> SMGYGNGVLIPHTPIAV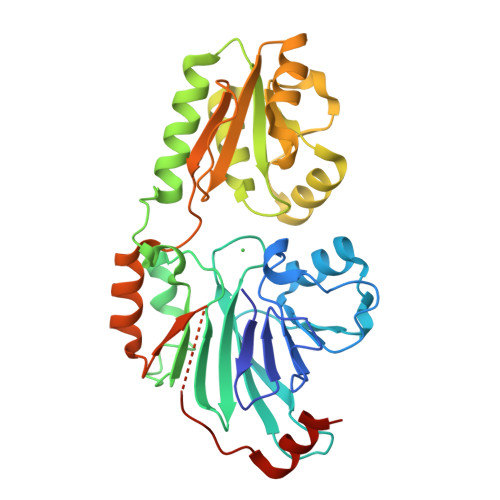DFWSLRRAGTARLFFLSHMHSDHTVGLSSTWARPLYCSPITAHLLHRYLQVSKQWIQALEVGESHVLPLDEIGQETMTVTLLDANHCPGSVMFLFEGYFGTILYTGDFRYTPSMLKEPALTLGKQIHTLYLDNTNCNPALVLPSRQEAAHQIVQLIRKHPQHNIKIGLYSLGKESLLEQLALEFQTWVVLSPRRLELVQLLGLADVFTVEEKAGRIHAVDHMEICHSNMLRWNQTHPTIAILPTSRKIHSSHPDIHVIPYSDHSSYSELRAFVAALKPCQVVPIVSRRPCGGFQDSLSPRISVPLIPDSVQQYMSSSSRKPS>MGDRGPEFVATTVELPLQQKADAAQTVTGPLPFGNSLLKEFVLDPAYRNLNHGSFGTIPSAIQQKLRSYQTAAEARPCPFLRYQTPVLLDESRAAVANLLKVPVETVVFVANATMGVNTVLRNIVWSADGKDEILYFDTIYGACGKTIDYVIEDKRGIVSSRCIPLIYPAEDDDVVAAFRDAIKKSREEGKRPRLAVIDVVSSMPGVRFPFEDIVKICKEEEIISCVDGAQGIGMVDLKITETDPDFLISNCHKWLFTPRGCAVFYVPVRNQHLIRSTLPTSHGFVPQVGNRFNPLVPAGNKSAFVSNFEFVGTVDNSPFFCVKDAIKWREEVLGGEERIMEYMTKLAREGGQKVAEILGTRVLENSTGTLIRCAMVNIALPFVVGEDPKAPVKLTEKEEKDVEGLYEIPHEEANMAFKWMYNVLQDEFNTFVPMTFHRRRFWARLSAQVYLEMSDFEWAGKTLKELCERVAKGEYKESALEVDLQGDHGLSAWSHPQFEK[8x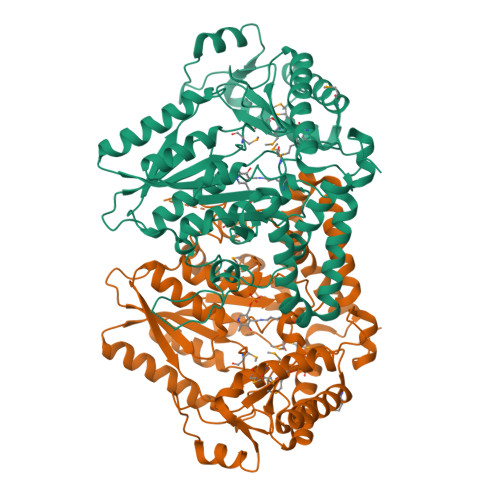]> GDRVADMIESSIGDSVSRALTQALPAPTGQNTQVSSHRLDTGEVPALQAAEIGASSNTSDESMIETRCVLNSHSTAETTLDSFFSRAGLVGEIDLPLEGTTNPSGYANWDIDITGYAQMRRKVELFTYMRFDAEFTFVACTPTGQVVPQLLQYMFVPPGAPKPESRESLAWQTATNPSVFVKLTDPPAQVSVPFMSPASAYQWFYDGYPTFGEHKQEKDLEYGACPNNMMGTFSVRTVGSSKSKYALVVRIYMRMKHVRAWIPRPMRNQNYLFKANPNYAGDSIKPTGTSRNAITTL;> SPSAEACGYSDRVAQLTIGNSTITTQEAANIIVGYGEWPSYCSDDDATAVDKPTRPDVSVNRFYTLDTKLWEKSSKGWYWKFPDVLTETGVFGQNAQFHYLYRSGFCIHVQCNASKFHQGALLVAILPEYVIGTVAGGTGTEDSHPPYIQTQPGADGFELQHPYVLDAGIPISQLTVCPHQWINLRTNNCATIIVPYMNTLPFDSALNHCNFGLLVVPISPLDFDQGATPVIPITITLAPMCSEFAGLRQAVTQ;> GFPTELKPGTNQFLTTDDGVSAPILPNFHPTPCIHIPGEVRNLLELCQVETILEVNNVPTNATSLME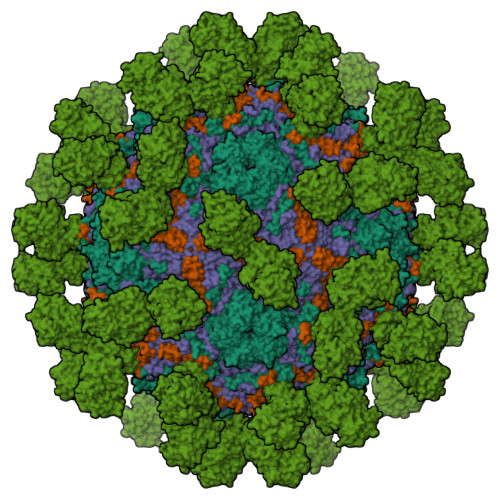RLRFPVSAQAGKGELCAVFRADPGRDGPWQSTMLGQLCGYYTQWSGSLEVTFMFTGSFMATGKMLIAYTPPGGPLPKDRATAMLGTHVIWDFGLQSSVTLVIPWISNTHYRAHARDGVFDYYTTGLVSIWYQTNYVVPIGAPNTAYIIALAAAQKNFTMKLCKDTSHILQTASIQ;> SHENSNSATEGSTINYTTINYYKDSYAATAGKQSLKQDPDKFANPVKDIFTEMAAPLK;> ETGVFQKAVDQSIEKKIVLRNGTEAFDSWEKPPLPVYTQFYFFNVTNPEEILRGETPRVEEVGPYTYRELRNKANIQFGDNGTTISAVSNKAYVFERDQSVGDPKIDLIRTLNIPVLTVIEWSQVHFLREIIEAMLKAYQQKLFVTHTVDELLWGYKDEILSLIHVFRPDISPYFGLFYEKNGTNDGDYVFLTGEDSYLNFTKIVEWNGKTSLDWWITDKCNMINGTDGDSFHPLITKDEVLYVFPSDFCRSVYITFSDYESVQGLPAFRYKVPAEILANTSDNAGFCIPEGNCLGSGVLNVSICKNGAPIIMSFPHFYQADERFVSAIEGMHPNQEDHETFVDINPLTGIILKAAKRFQINIYVKKLDDFVETGDIRTMVFPVMYLNESVHIDKETASRLKSMINTTGKHHHHHH> MRLKVMMDVNKKTKIRHRNELNHTLAQLPLPAKRVMYMALALIDSKEPLERGRVFKIRAEDLAALAKITPSLAYRQLKEGGKLLGASKISLRGDDIIALA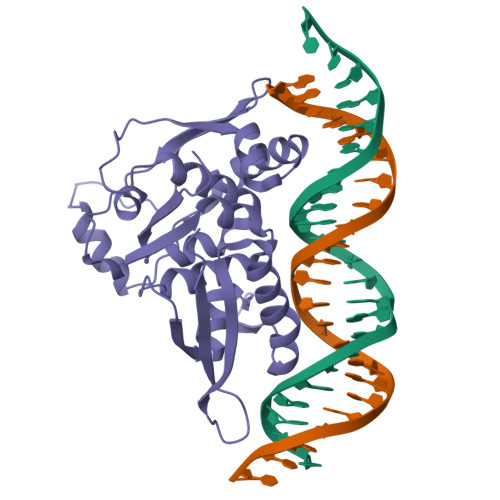KELNLLSTAKNSSEELDLNIIEWIAYSPDEGYLSLKFTRTIEPYISSLIGKKNKFTTQLLTASLRLSSQYSSSLYQLIRKHYSNFKKKNYFIISVDELKEELIAYTFDKDGNIEYKYPDFPIFKRDVLNKAIAEIKKKTEISFVGFTVHEKEGRKISKLKFEFVVDEDEFSGDKDD>MHVTLVEINVKEDKVDQFIEVFRANHLGSIREAGNLRFDVLRDEHIPTRFYIYEAYTDEAAVAIHKTTPHYLQCVEQLAPLMTGPRKKT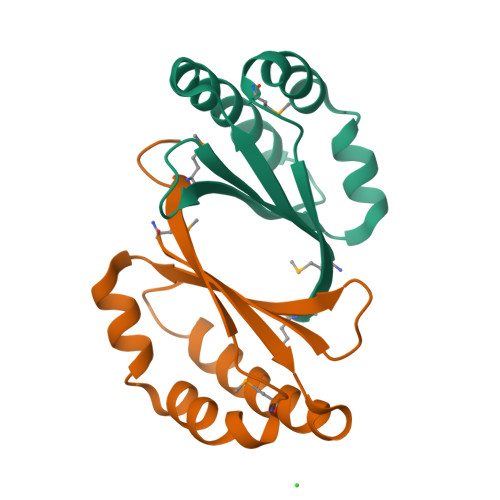VFIGLMPGSLEHHHHHH[2x]> MTRAEVGLVWA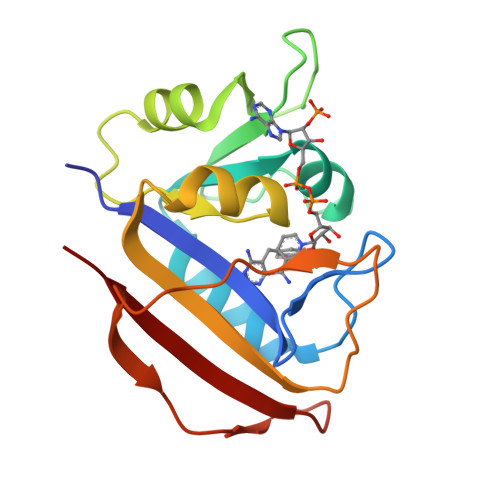QSTSGVIGRGGDIPWSVPEDLTRFKEVTMGHTVIMGRRTWESLPAKVRPLPGRRNVVVSRRPDFVAEGARVAGSLEAALAYAGSDPAPWVIGGAQIYLLALPHATRCEVTEIEIDLRRDDDDALAPALDDSWVGETGEWLASRSGLRYRFHSYRRD MERCAPTOMETHYL 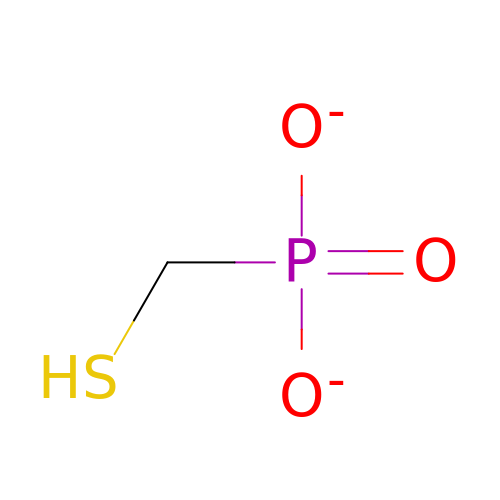PHOSPHONATE | C H3 O3 P S | MJZCELCYTRONIX-UHFFFAOYSA-L>SMLLQGKVALITGAASERGIGRATAEIFAQQGAKVIIVDLDLAQSQNAAKALGEGHMGLAANVANEEQVKAAVEQALQHYGKIDILINNAGITQPIKTLDIQRSDYDRVLDVSLRGTLIMSQAVIPSMKANGGGSIVCL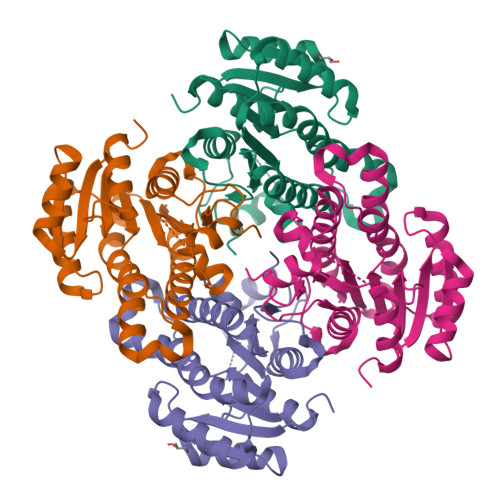SSVSAQRGGGIFGGPHYSAAKAGVLGLAKAMAREFGGDQIRVNSLTPGLIQTDITGGLMNDDRRHDILAGIPLGRLGKAQDVANAALFLASDLSAYLTGVTLDVNGGMLIH[4x]> MAVKVEYDLKRLRNIGIAAHIDAGKTTTTERILYYTGRIHKIGEVHEGAATMDFMEQERERGITITAAVTTCFWKDHRINIIDTPGHVDFTIEVERSMRVLDGAIVVFDSSQGVEPQSETVWRQAEKYKVPRIAFANKMDKTGADLWLVIRTMQERLGARPVVMQLPIGREDTFSGIIDVLRMKAYTYGNDLGTDIREIPIPEEYLDNAREYHEKLVEVAADFDENIMLKYLEGEEPTEEELVAAIRKGTIDLKITPVFLGSALKNKGVQLLLDAVVDYLPSPLDIPPIKGTTPEGEVVEIHPDPNGPLAALAFKIMADPYVGRLTFIRVYSGTLTSGSYVYNTTKGRKERVARLLRMHANHREEVEELKAGDLGAVVGLKETITGDTLVGEDAPRVILESIEVPEPVIDVAIEPKTKADQEKLSQALARLAEEDPTFRVSTHPETGQTIISGMGELHLEIIVDRLKREFKVDANVGKPQVAYRETITKPVDVEGKFIRQTGGRGQYGHVKIKVEPLPRGSGFEFVNAIVGGVIPKEYIPAVQKGIEEAMQSGPLIGFPVVDIKVTLYDGSYHEVDSSEMAFKIAGSMAIKEAVQKGDPVILEPIMRVEVTTPEEYMGDVIGDLNARRGQILGMEPRGNAQVIRAFVPLA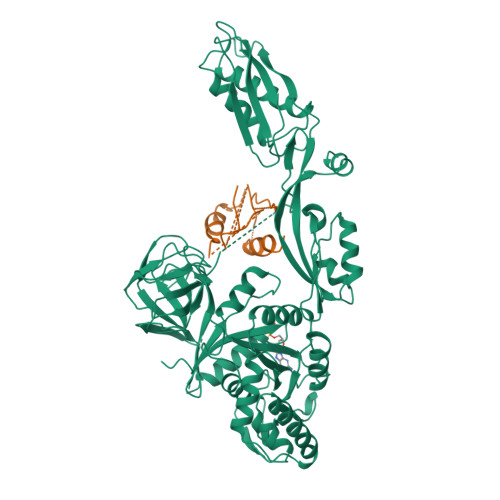EMFGYATDLRSKTQGRGSFVMFFDHYQEVPKQVQEKLIKGQ>GPEIPQGVLSVDSAMPMVLHLLAPLAAKFNERYPHIRLSLVSSEGYINLIERKVDIALRAGELDDSGLRARHLFDSRFRVIASPEYLAKHGTPQSTEELAGHQCLGFTEPGSLNTWAVLDAQGNPYKISPHFTASSGEILRSLCLSGCGIVCLSDFLVDNDIAEGKLIPLLAEQTSDKTHPFNAVYYSDK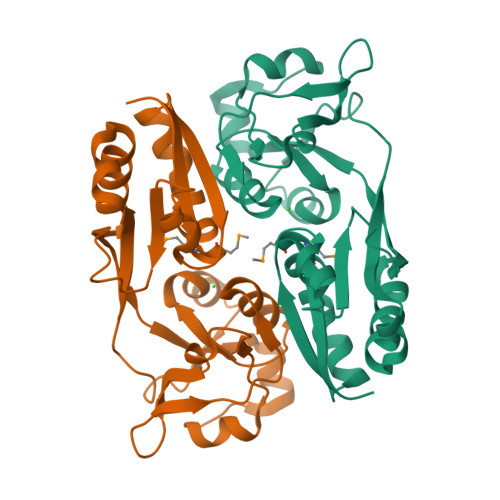AVNLRLRVFLDFLVEELGNNLCG[2x]>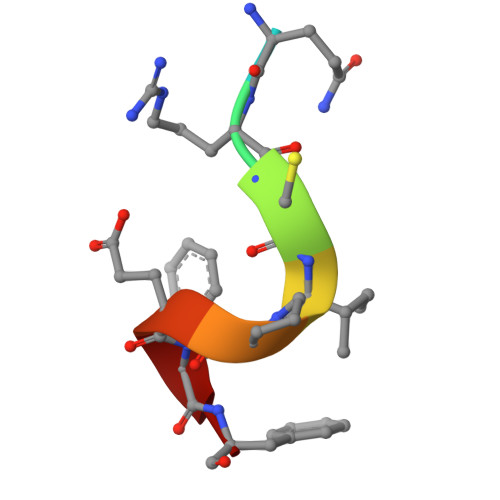 SQRCIPEFF>[2x]MVEMGRREEMIAKIKELMLQPERIRNIGIAAHIDHGKTTLSDNLLAGAGMISEELAGKQLVLDFDEQEQARGITINAANVSMVHNYEGKDYLINLIDTPGHVDFGGDVTRAMRAIDGVIIVVDAVEGVMPQTETVVRQALREYVKPVLFINKVDRLIRELKLTPQQMMERFSKIIMDVNRLIQRYAPEEYKKKWMVKVEDGSVAFGSAYYNWALSVPFMKRTGVKFNEIIDLTLKGDN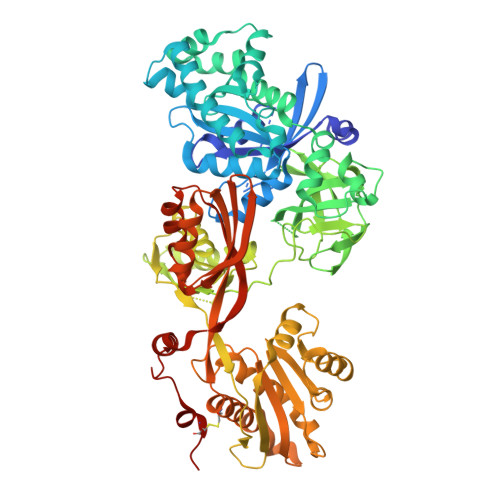RTLRQKAPLHVVVLDMVVRHLPSPIEAQKYRIPHLWEGDISSDIGQAMLNCDPKGKMVMVVTKIIIDKHAGEVATGRVWSGTVKSGQEVYLINTKRKARIQQVGIYMGPERINMEAVPAGNIVAVTGLRDAMAGETVAEEQIEPFEALHYVSEPVVTVAIEAKNVKDLPRLIEALRQLAKEDPTLHVKIDEETGQHLLSGMGELHLEVKLYKLKKDWGIDIEVSEPIVVYRESITKSSPMVEGKSPNRHNRFYIVVEPMPDEIYNAIKEGIIPEGRVKNPKEVAKKLAELGMDYEIARGIVDIYNGNMFIDNTKGVQYLNEVMDLLIDGFHQAMDEGPLAREPVMKVIVRLLDAQVHEDNVHRGPAQIYPAIRTAIHCAMMKSNPVLYEPYQKVIINIPYEYMGAVSREITQRRGQLVDMKQEGEVMTIIAEAPVAEMFGFAGSIRSATSGRALWSTEHAGFKRVPNELAQQIIRQIRQRKGLDPNPPTEKDVCPLFLEHHHHHH> EETVTCLQMTVYHPGQLQCGIFQSISFNREKLPSSEVVKFGRNSNICHYTFQDKQVSRVQFSLQLFKKFNSSVLSFEIKNMSKKTNLIVDSRELGYLNKMDLPYRCMVRFGEYQFLMEKEDGESLEFFETQF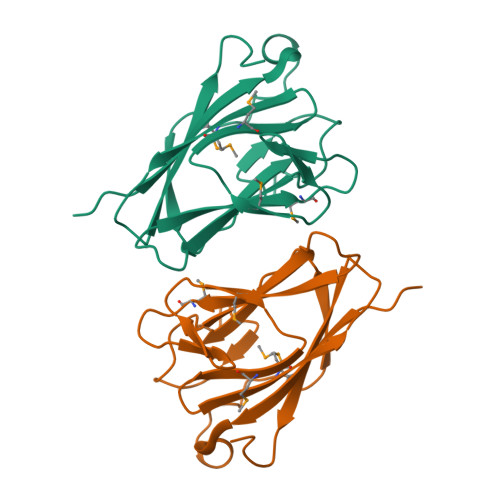ILSPRSLL methyl 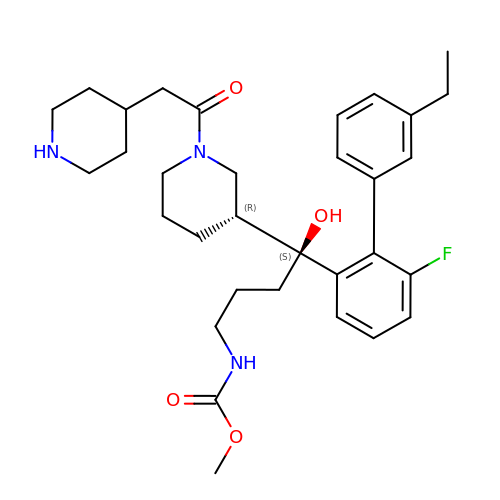[(4S)-4-(3'-ethyl-6-fluoro[1,1'-biphenyl]-2-yl)-4-hydroxy-4-{(3R)-1-[(piperidin-4-yl)acetyl]piperidin-3-yl}butyl]carbamate | C32 H44 F N3 O4 | WBSHAODYCYXPAY-DICHSLLOSA-N According to their amino acid sequences, β-lactamases are classified into class A, C, and D enzymes, which utilize serine for β-lactam hydrolysis (SBLs), and class B metalloenzymes (MBLs), which require divalent zinc ions for substrate hydrolysis. AmpC β-lactamases are clinically relevant cephalosporinases. They mediate resistance to cephalothin, cefazolin, cefoxitin, most penicillins, and to β-lactamase inhibitor (BLI)-β-lactam combinations. In many bacteria, AmpC enzymes are inducible and can be over-expressed by mutation thus extending resistance to broad-spectrum cephalosporins i.e. cefotaxime, ceftazidime, and ceftriaxone.

Inhibitor 3 is covalently bound through the boron atom to the side chain oxygen atom (Oγ) of Ser64, adopting a tetrahedral geometry as already reported for other similar complexes. The catalytic and conserved residues in AmpC β-lactamase catalytic domain undergo minimal rearrangements upon binding. The boronic acid oxygen atom O13 forms strong hydrogen bonds with the −OH group of the side chain Tyr150 and with a water molecule W567, commonly highly conserved in AmpC binary complexes with aryl boronic acid inhibitors. The meta carboxyvinyl lateral chain of the ligand molecule is placed near Tyr221 and is stabilized by the π⋅⋅⋅H−C interaction. In class C SBLs, the carboxylate group does not interact in the typical carboxylate site of antibiotics as in class A SBLs, but, on the contrary, is oriented in the opposite direction, towards Asn152, Gln120, and Leu119, where usually the R1 chain of antibiotics binds. The major structural change involves the region near the phenyl ring of compound 3 and comprises a conformational shift of the side chain residues Gln120 and Asn152. Comparing to the structure of native PaAmpC, in the crystal structure of PaAmpC: 3 the side chain of Gln120 is rotated by 50 degrees and the side chain of the Asn152 accommodates a flipped orientation and show a shift of 36 degrees. In contrast, in the PaAmpC:3 complex the inhibitor points its meta carboxyvinyl group towards the opposite direction, extensively interacting with the aqueous solvent. Compounds 3 and 5 do not experience improvement in affinity compared to lead phenylboronic acid 1, thus reflecting the lack of strong additional specific interactions for meta derivatives in AmpC binding site.

> MRDTRFPCLCGIAASTLLFATTPAIAGEAPADRLKALVDAAVQPVMKANDIPGLAVAISLKGEPHYFSYGLASKEDGRRVTPETLFEIGSVSKTFTATLAGYALTQDKMRLDDRASQHWPALQGSRFDGISLLDLATYTAGGLPLQFPDSVQKDQAQIRDYYRQWQPTYAPGSQRLYSNPSIGLFGYLAARSLGQPFERLMEQQVFPALGLEQTHLDVPEAALAQYAQGYGKDDRPLRVGPGPLDAEGYGVKTSAADLLRFVDANLHPERLDRPWAQALDATHRGYYKVGDMTQGLGWEAYDWPISLKRLQAGNSTPMALQPHRIARLPAPQALEGQRLLNKTGSTNGFGAYVAFVPGRDLGLVILANRNYPNAERVKIAYAILSGLEQQGKVPLKR> MAFSATLSQLSSLSTISSSLPISSRRLPHRSLPQFTVKAEAEKEKQSAQAKSDGEASPAATKTPKTLPKKPVYSMKKGQIVRVEKEKYLNSINYLSVGHPPFYKGLDYIYEDRGEVLDLRVFE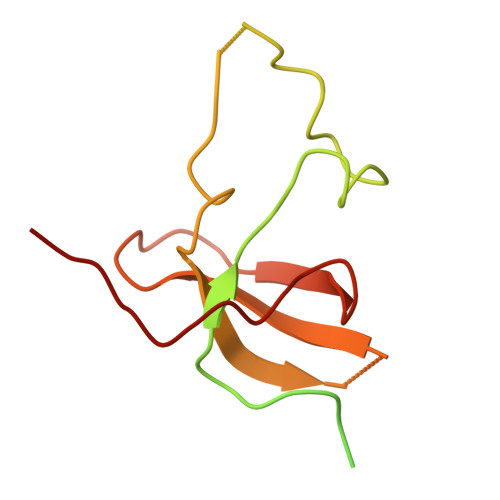TGEYALVGWVGIPTAPAWLPTDMLIKCEKLVYERM>[4x]MH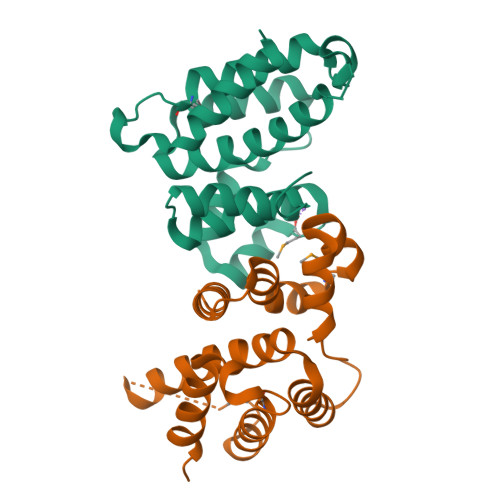HHHHHMYEKARQMMIEAHSGQVRKITGEPYFSHPLNVARILRRAGFREEVVVAGLLHDAVEDTEMTDADIRATFGDEVADLVASHTENKTLSWEERKAHTIEQVRTGNLEEKALIVADKLDNLTSVKYALSSEGKSVWSYFKRGYDLQKWYNQGIKNNMEYGLNPSEIPPFFDEYARLVKWIFKK>[3x]GHHHHHHELANNTTGFTRIIKAAGYSWKGLRAAWINEAAFRQEGVAVLLAVVIACWLDVDACTRVLLISSVMLVMIVELLNSAIEAVVDRIGSEYHELSGRAKDLGSAAVLIAIIDAVITWCILLWSHFG

Diacylglycerol kinase (DgkA) is the smallest known kinase. In Escherichia coli, it is responsible for the adenosine triphosphate (ATP)-dependent phosphorylation of diacylglycerol (DAG) to phosphatidic acid used in periplasm membrane-derived oligosaccharide synthesis in response to osmotic shock1. The enzyme has long served as a model for integral membrane enzymology, folding456, assembly and stability. It is a trimer with three active sites of the shared sites type that exhibits moderate positive heteroallostery, random-binding kinetics and lipid substrate promiscuity. Each subunit has four helices, three of which are largely membrane embedded (H1-3), whereas the fourth, an N-terminal amphiphilic surface helix (SH), anchors the protein at the membrane interface.

However, in our studies of DgkA to date, we have crystal structures that include a total of 10 trimers with density in the active site for bound lipid that is variable (refs 12, 17 and this work). Mapping these onto a single active site makes a convincing case that lipids reside in the binding pocket. Their variable definition likely reflects acyl chain flexibility and lipid movement during reaction.> MVGRMMATAPATAADVKQVGYVQQIIGAVVDVTFTDSVPPVLTALTVDAKETGTLLTMEIVQHLDTKTARCICMSSTDMLRLRTPVVNTGSQITVPVGEATLGRIFNVMGDAIDQRGPVKNKVRWPIHRKAPTLAEQSGKDEVLVTGIKVIDLILPYCKGGKIGLFGGAGVGKTVIIMELINNVAKGHGGYSVFAGVGERTREGTDLYLEMMGSKVIDLQGDSKC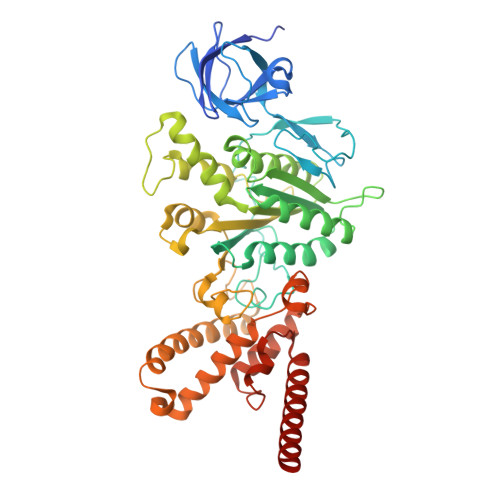VLVYGQMNEPPGARARVAQTALTMAEYFRDEAGQDVLLFVDNVFRFTQANSEVSALLGRIPAAVGYQPTLAEDLGMLQERITSTVKGSITSVQAVYVPADDITDPAPATTFSHLDATTVLSRSVAEAGIYPAVEPLECASRIMDPDAIDVNHYNVAMDIVEMLTKYKELQDIIAVLGIDELSEEDKLIVDRARKVAKFMSQPFAVAEVFTGMKGYYVQLEDCVSDFGSLLMGQCDNIPEMAFYMVGGLDSVKEKAAKMAAEAAAMRERARKAAEAK>MSKLIVPQWPLPKGVAACSSTRIGGVSLPPYDSLNLGAHCGDNPDHVEENRKRLFAAGNLPSKPVWLEQVHGKDVLKLTGEPYASKRADASYSNTPGTVCAVMTADCLPVLFCNRAGTEVAAVHAGWRGLCAGVLEETVSCFADKPENILAWLGPAIGPRAFEVGAEVREAFMAVDAKASAAFIQHGDKYLADIYQLARQRLANVGVEQI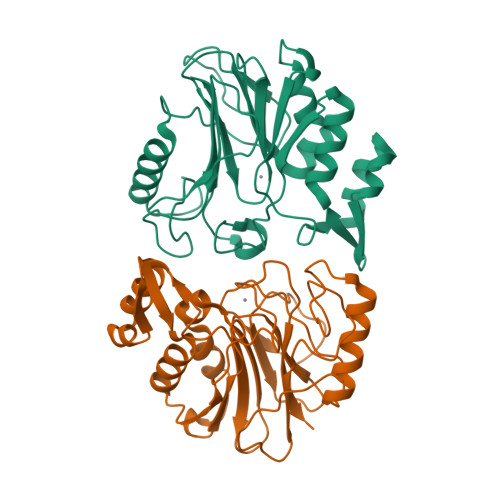FGGDRCTYTENETFFSYRRDKTTGRMASFIWLI[2x]>[6x]AAPSFDCGKPQVEPKKCP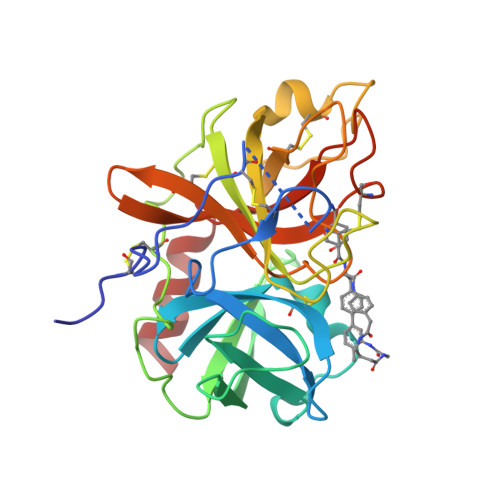GRVVGGCVAHPHSWPWQVSLRTRFGMHFCGGTLISPEWVLTAAHCLEKSPRPSSYKVILGAHQEVNLEPHVQEIEVSRLFLEPTRKDIALLKLSSPAVITDKVIPACLPSPNYVVADRTECFITGWGETQGTFGAGLLKEAQLPVIENKVCNRYEFLNGRVQSTELCAGHLAGGTDSCQGDSGGPLVCFEKDKYILQGVTSWGLGCARPNKPGVYVRVSRFVTWIEGVMRNN>[2x]MSMLVVVTENVPPRLRGRLAIWLLEVRAGVYVGDVSA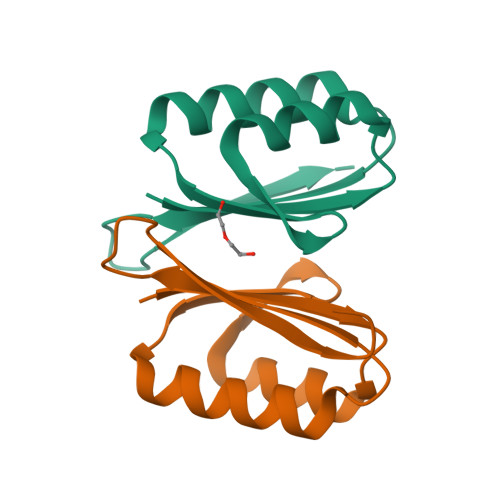KIREMIWEQIAGLAEEGNVVMAWATNTETGFEFQTFGLNRRTPVDLDGLRLVSFLPV> MKVLYFAEIKDILQKAQEDI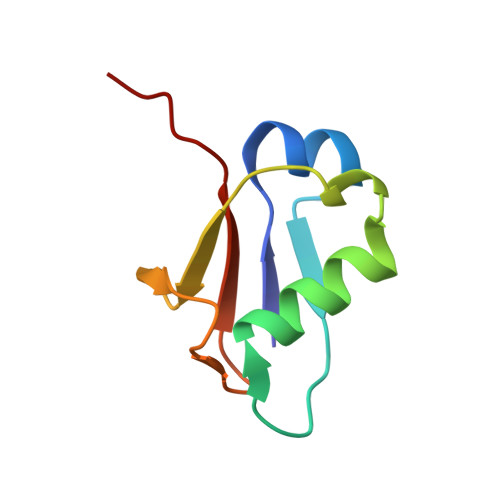VLEQALTVQQFEDLLFERYPQINNKKFQVAVNEEFVQKSDFIQPNDTVALIPPVSGG> MMRYRKGARDTAFLVLYRWDLRGENPGELFKEVVEEKNIKNKDAYEYAKKLVDTAVRHIEEIDSIIEK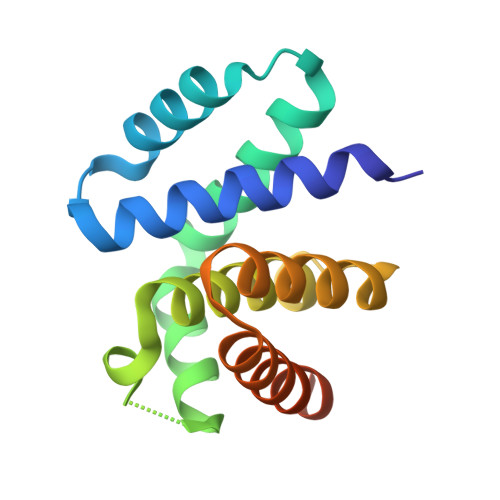HLKGWSIDRLGYVERNALRLGVAELIFLKSKEPGRVFIDIVDLVKKYADEKAGKFVNGVLSAIYKAYITSSKEEKPSLKSE> MVSPTKMIIRSPLKETDTNLKHNNGIAASTTAAGHLNVFSNDNNCNNNNTTESFPKKRSLERLELQQQQHLHEKKRARIERARSIEGAVQVSKGTGLKNVEPRVTPKELLEWQTNWKKIMKRDSRIYFDITDDVEMNTYNKSKMDKRRDLLKRGFLTLGAQITQFFDTTVTIVITRRSVENIYLLKDTDILSRAKKNYMKVWSYEKAARFLKNLDVDLDHLSKTKSASLAAPTLSNLLHNEKLYGPTDRDPRTKRDDIHYFKYPHVYLYDLWQTWAPIITLEWKPQELTNLDELPYPILKIGSFGRCPFIGDRNYDESSYKRVVKRYSRDKANKKYALQLRALFQYHADTLLNTSSVNDQTKNLIFIPHTCNDSTKSFKKWMQEKAKNFEKTELKKTDDSAVQDVRNEHADQTDEKNSILLNETETKEPPLKEEKENKQSIAEESNKYPQRKELAATPKLNHPVLATFARQETEEVPDDLCTLKTKSRQAFEIKASGAHQSNDVATSFGNGLGPTRASVMSKNMKSLSRLMVDRKLGVKQTNGNNKNYTATIATTAETSKENRHRLDFNALKKDEAPSKETGKDSAVHLETNRKPQNF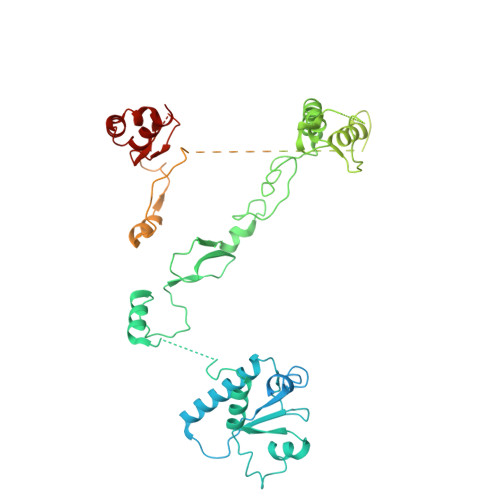PKVATKSVSADSKVHNDIKITTTESPTASKKSTSTNVTLHFNAQTAQTAQPVKKETVKNSGYCENCRVKYESLEQHIVSEKHLSFAENDLNFEAIDSLIENLRFQI> GSHMAEDEPFSGAKKLRHLLENTDELIVCPGVYDGLSARTAMELGFKSLYMTGAGTTASRLGQPDLAIAQLHDMRDNADMIANLDPFGPPLIADMDTGYGGPIMVARTVEHYIRSGVAGAHLEDQILTKRCGHLSGKKVVSRDEYLVRIRAAVAT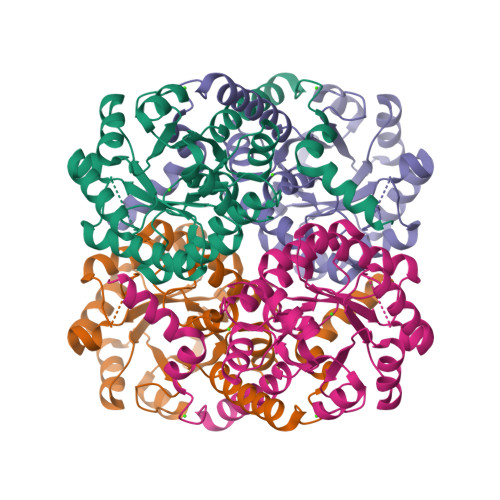KRRLRSDFVLIARTDALQSLGYEECIERLRAARDEGADVGLLEGFRSKEQAAAAVAALAPWPLLLNSVENGHSPLITVEEAKAMGFRIMIFSFATLAPAYAAIRETLVRLRDHGVVGTPDGITPVRLFEVCGLQDAMEVDNGAGGKAFSEGV>[4x]MSKATYKERAATHPSPVAAKLFNIMHEKQTNLCASLDVRTTKELLELVEALGPKICLLKTHVDILTD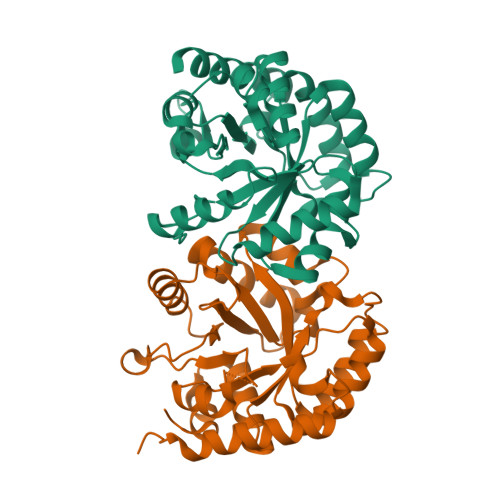FSMEGTVKPLKALSAKYNFLLFENRKFADIGNTVKLQYSAGVYRIAEWADITNAHGVVGPGIVSGLKQAAEEVTKEPRGLLMLAELSCKGSLATGEYTKGTVDIAKSDKDFVIGFIAQRDMGGRDEGYDWLIMTPGVGLDDKGDALGQQYRTVDDVVSTGSDIIIVGRGLFAKGRDAKVEGERYRKAGWEAYLRRCGQQN> ALSEIETRHSEIIKLENSIRELHDMFMDMAMLVESQGEMIDRIEYNVEHAVDYVERAVS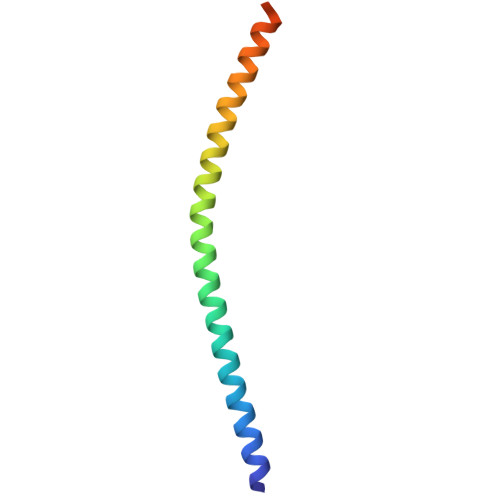DTKKAVKYQSKARRKKIM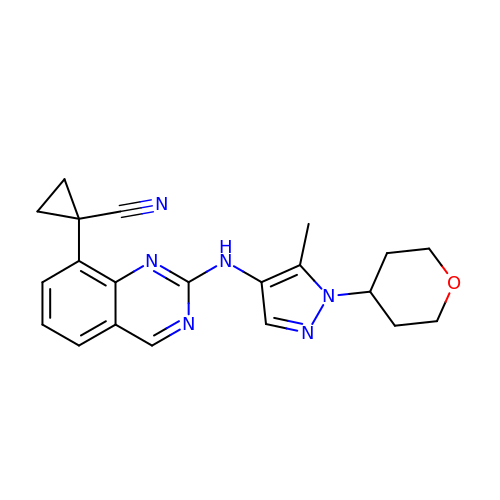1-(2-{[5-methyl-1-(oxan-4-yl)-1H-pyrazol-4-yl]amino}quinazolin-8-yl)cyclopropane-1-carbonitrile | C21 H22 N6 O | NSRPXCKUNCQCDO-UHFFFAOYSA-N>[4x]TLQESDKFATKAIHAGEHVDVHGSVIEPISLSTTFKQSSPANPIGTYEYSRSQNPNRENLERAVAALENAQYGLAFSSGSATTATILQSLPQGSHAVSIGDVYGGTHRYFTKVANAHGVETSFTNDLLNDLPQL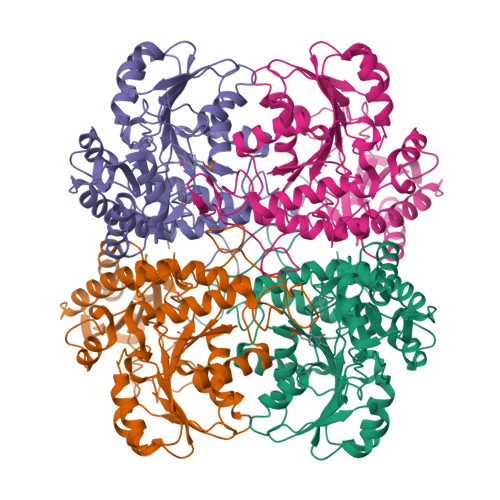IKENTKLVWIETPTNPTLKVTDIQKVADLIKKHAAGQDVILVVDNTFLSPYISNPLNFGADIVVHSATKYINGHSDVVLGVLATNNKPLYERLQFLQNAIGAIPSPFDAWLTHRGLKTLHLRVRQAALSANKIAEFLAADKENVVAVNYPGLKTHPNYDVVLKQHRDALGGGMISFRIKGGAEAASKFASSTRLFTLAESLGGIESLLEVPAVMTHGGIPKEAREASGVFDDLVRISVGIEDTDDLLEDIKQALKQATN>[4x]MSLEDKDLRSIQEVRNLIESANKAQKELAAMSQQQIDTIVKAI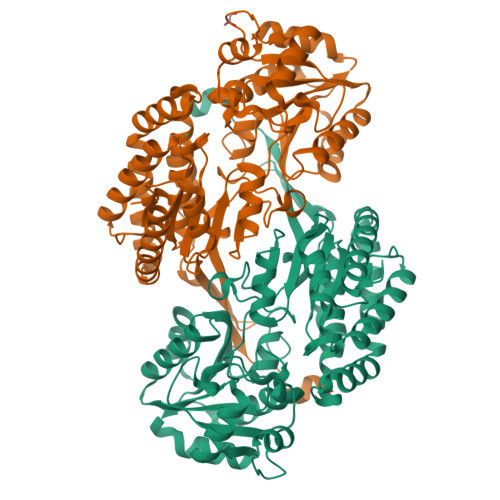ADAGYGAREKLAKMAHEETGFGIWQDKVIKNVFASKHVYNYIKDMKTIGMLKEDNEKKVMEVAVPLGVVAGLIPSTNPTSTVIYKTLISIKAGNSIVFSPHPNALKAILETVRIISEAAEKAGCPKGAISCMTVPTIQGTDQLMKHKDTAVILATGGSAMVKAAYSSGTPAIGVGPGNGPAFIERSANIPRAVKHILDSKTFDNGTICASEQSVVVERVNKEAVIAEFRKQGAHFLSDAEAVQLGKFILRPNGSMNPAIVGKSVQHIANLAGLTVPADARVLIAEETKVGAKIPYSREKLAPILAFYTAETWQEACELSMDILYHEGAGHTLIIHSEDKEIIREFALKKPVSRLLVNTPGALGGIGATTNLVPALTLGCGAVGGSSSSDNIGPENLFNIRRIATGVLELEDIREGHHHHHH>MDLFSVRMRAQKNGKHVSGAERIVKKEELETAVKELLNRPKEFDFMNVKVEKVKDFEVVKFNLKISTYSFKSPEEAREFAVKKLTQEGIKEEVAKKAVEILSKGANPKGGNMRGAVLMDIETGERLEEDKERGVRTIHFDWKDRKKVTEKLLKEGYTLRTVDALALTFKNLFCGVVAELCWSDDPDYVTGYVS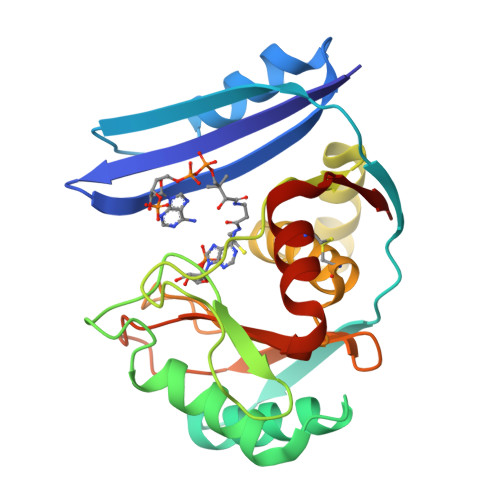GKEIGYVRITPLKEKGDPLGGRVYFVSRKELSEIIECLTQKVVLIEL[2x]> MEKETGPEVDDSKVTYDTIQSKVLKAVIDQAFPRVKEYSLNGHTLPGQVQQFNQVFINNHRITPEVTYKKINETTAEYLMKLRDDAHLINAEMTVRLQVVDNQLHFDVTKIVNHNQVTPGQKIDDESKLLSSISFLGNALVSVSSDQTGAKFDGATMSNNTHVSGDDHIDVTNPMKDLAKGYMYGFVSTDKLAAGVWSNSQNSYGGGSNDWTRLTAYKETVGNANYVGIHSSEWQWEKAYKGIVFPEYTKELPSAKVVITEDANADKNVDWQDGAIAYRSIMNNPQGWEKVKDITAYRIAMNFGSQAQNPFLMTLDGIKKINLHTDGLGQGVLLKGYGSEGHDSGHLNYADIGKRIGGVEDFKTLIEKAKKYGAHLGIHVNASETYPESKYFNEKILRKNPDGSYSYGWNWLDQGINIDAAYDLAHGRLARWEDLKKKLGDGLDFIYVDVWGNGQSGDNGAWATHVLAKEINKQGWRFAIEWGHGGEYDSTFHHWAADLTYGGYTNKGINSAITRFIRNHQKDAWVGDYRSYGGAANYPLLGGYSMKDFEGWQGRSDYNGYVTNLFAHDVMTKYFQHFTVSKWENGTPVTMTDNGSTYKWTP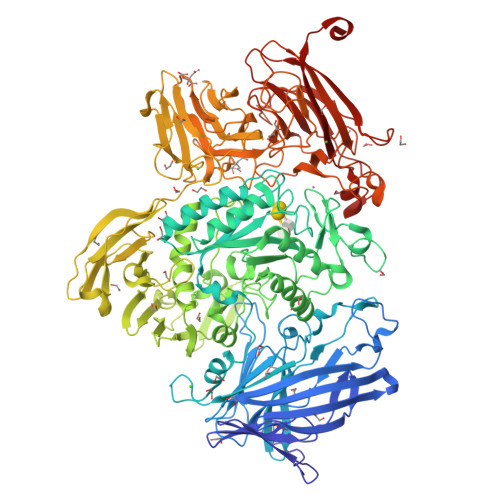EMRVELVDADNNKVVVTRKSNDVNSPQYRERTVTLNGRVIQDGSAYLTPWNWDANGKKLSTDKEKMYYFNTQAGATTWTLPSDWAKSKVYLYKLTDQGKTEEQELTVKDGKITLDLLANQPYVLYRSKQTNPEMSWSEGMHIYDQGFNSGTLKHWTISGDASKAEIVKSQGANDMLRIQGNKEKVSLTQKLTGLKPNTKYAVYVGVDNRSNAKASITVNTGEKEVTTYTNKSLALNYVKAYAHNTRRNNATVDDTSYFQNMYAFFTTGADVSNVTLTLSREAGDEATYFDEIRTFENNSSMYGDKHDTGKGTFKQDFENVAQGIFPFVVGGVEGVEDNRTHLSEKHDPYTQRGWNGKKVDDVIEGNWSLKTNGLVSRRNLVYQTIPQNFRFEAGKTYRVTFEYEAGSDNTYAFVVGKGEFQSGRRGTQASNLEMHELPNTWTDSKKAKKATFLVTGAETGDTWVGIYSTGNASNTRGDSGGNANFRGYNDFMMDNLQIEEITLTGKMLTHHHHHH> MTVRKNQATLTADEKRRFVAAVLELKRSGRYDEFVRTHNEFIMSDTDSGERTGHRSPSFLPWHRRFLLDFEQALQSVDSSVTLPYWDWSADRTVRASLWAPDFLGGTGRSTDGRVMDGPFAASTGNWPINVRVDSRTYLRRSLGGSVAELPTRAEVESVLAISAYDLPPYNSASEGFRNHLEGWRGVNLHNRVHVWVGGQMATGVSPNDPVFWLHHAYVDKLWAEWQRRHPDS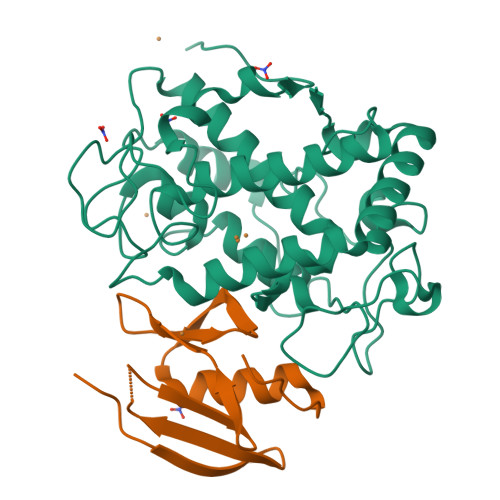AYVPTGGTPDVVDLNETMKPWNTVRPADLLDHTAYYTFDALEHHHHHH;> MPEITRRRALTAAAAVAATASAAVTLAAPAASAAGHHEPAAPESFDEVYKGRRIQGRPAGGGAHHHEHGGGYEVFVDGVQLHVLRNADGSWISVVSHYDPVPTPRAAARAAVDELQGAPLLPFPANLEHHHHHH> NSVLFPCKYASSGCEITLPHTEKAEHEELCEFRPYSCPCPGASCKWQGSLDAVMPHLMHQHKSITTLQGEDIVFLATDINLPGAVDWVMMQSCFGFHFMLVLEKQEKYDGHQQFFAIVQLIGTRKQAENFAYRLELNGHRRRLTWEATPRSIHEGIATAIMNSDCLVFDT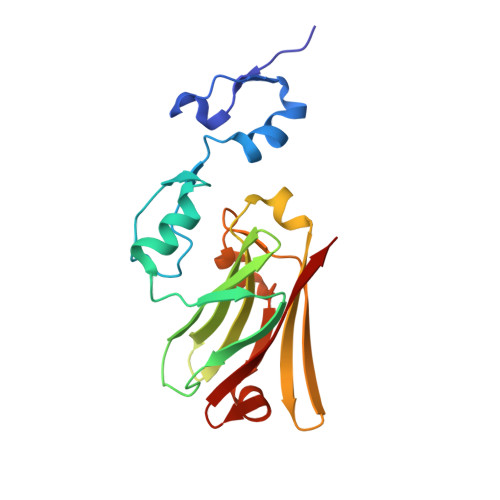SIAQLFAENGNLGINVTISMC> HAADRIARLPGQPAVDFDMYSGYITVDEGAGRSLFYLLQEAPEDAQPAPLVLWLNGGPGCSSVAYGASEELGAFRVKPRGAGLVLNEYRWNKVANVLFLDSPAGVGFSYTNTSSDIYTSGDNRTAHDSYAFLAKWFERFP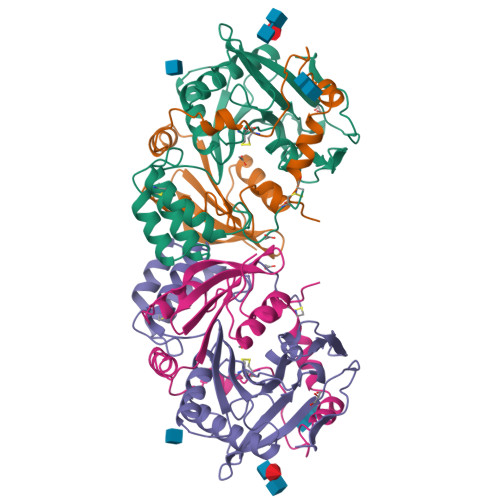HYKYRDFYIAGESYAGHYVPELSQLVHRSKNPVINLKGFMVGNGLIDDYHDYVGTFEFWWNHGIVSDDTYRRLKEACLHDSFIHPSPACDAATDVATAEQGNIDMYSLYTPVCNI;> SYDPCTERYSTAYYNRRDVQMALHANVTGAMNYTWATCSDTINTHWHDAPRSMLPIYRELIAAGLRIWVFSGDTDAVVPLTATRYSIGALGLPTTTSWYPWYDDQEVGGWSQVYKGLTLVSVRGAGHEVPLHRPRQALVLFQYFLQGKPMPGQ>MEIYEGKLTAEGLRFGIVASRFNHALVDRLVEGAIDCIVRHGGREEDITLVRVPGSWEIPVAAGELARKEDIDAVIAIGVLIRGATPHFDYIASEVSKGLANLSLELRKPITFGVITADTLEQAIERAGTKHGNKGWEAALSAIEMA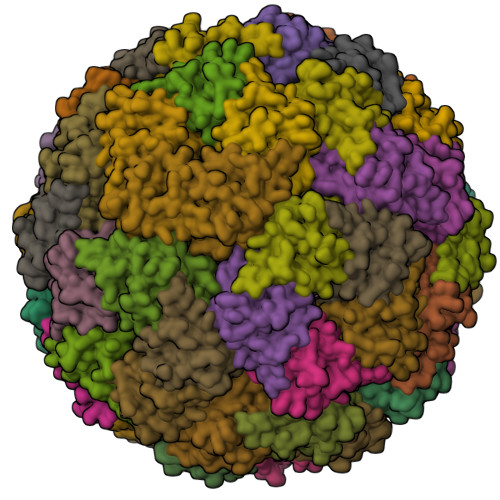NLFKSLR[60x]> MKDLLKFLKAQTKTEEFDAIKIALASPDMIRSWSFGEVKKPETINYRTFKPERDGLFCARIFGPVKDYECLCGKYKRLKHRGVICEKCGVEVTQTKVRRERMGHIELASPTAHIWFLKSLPSRIGLLLDMPLRDIERVLYFESYVVIEGGMTNLERQQILTEEQYLDALEEFGDEFDAKMGAEAIQALLKSMDLEQECEQLREELNETNSETKRKKLTKRIKLLEAFVQSGNKPEWMILTVLPVLPPDLRPLVPLDGGRFATSDLNDLYRRVINRNNRLKRLLDLAAPDIIVRNEKRMLQEAVDALLDNGRRGRAITGSNKRPLKSLADMIKGKQGRFRQNLLGKRVDYSGRSVITVGPYLRLHQCGLPKKMALELFKPFIYGKLELRGLATTIKAAKKMVEREEAVVWDILDEVIREHPVLLNRAPTLHRLGIQAFEPVLIEGKAIQLHPLVCAAYNADFDGDQMAVHVPLTLEAQLEARALMMSTNNILSPANGEPIIVPSQDVVLGLYYMTRDCVNAKGEGMVLTGPKEAERLYRSGLASLHARVKVRITEYEKDANGELVAKTSLKDTTVGRAILWMIVPKGLPYSIVNQALGKKAISKMLNTCYRILGLKPTVIFADQIMYTGFAYAARSGASVGIDDMVIPEKKHEIISEAEAEVAEIQEQFQSGLVTAGERYNKVIDIWAAANDRVSKAMMDNLQTETVINRDGQEEKQVSFNSIYMMADSGARGSAAQIRQLAGMRGLMAKPDGSIIETPITANFREGLNVLQYFISTHGARKGLADTALKTANSGYLTRRLVDVAQDLVVTEDDCGTHEGIMMTPVIEGGDVKEPLRDRVLGRVTAEDVLKPGTADILVPRNTLLHEQWCDLLEENSVDAVKVRSVVSCDTDFGVCAHCYGRDLARGHIINKGEAIGVIAAQSIGEPGTQLTMRTFHIGGAASRAAAESSIQVKNKGSIKLSNVKSVVNSSGKLVITSRNTELKLIDEFGRTKESYKVPYGAVLAKGDGEQVAGGETVANWDPHTMPVITEVSGFVRFTDMIDGQTITRQTDELTGLSSLVVLDSAERTAGGKDLRPALKIVDAQGNDVLIPGTDMPAQYFLPGKAIVQLEDGVQISSGDTLARIPQESGGTKDITGGLPRVADLFEARRPKEPAILAEISGIVSFGKETKGKRRLVITPVDGSDPYEEMIPKWRQLNVFEGERVERGDVISDGPEAPHDILRLRGVHAVTRYIVNEVQDVYRLQGVKINDKHIEVIVRQMLRKATIVNAGSSDFLEG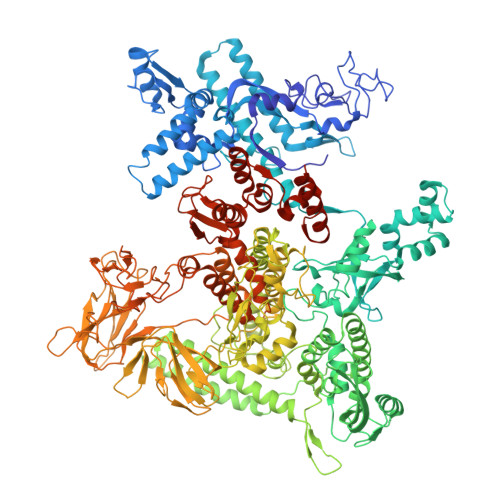EQVEYSRVKIANRELEANGKVGATYSRDLLGITKASLATESFISAASFQETTRVLTEAAVAGKRDELRGLKENVIVGRLIPAGTGYAYHQDRMRRRAAGEAPAAPQVTAEDASASLAELLNAGLGGSDNE> YVEFVAQISPQYPMFTVPLPIPPVKQPRLTVTNPVNGQEIWYYEVEIKPFTHQVYPDLGSADLVGYDGMSPGPTFQVPRGVETVVRFINNAEAPNSVHLHGSFSRAAFDGWAEDITEPGSFKDYYYPNRQSARTLWYHDHAMHITAENAYRGQAGLYMLTDPAEDALNLPSGYGEFDIPMILTSKQYTANGNLVTTNGELNSFWGDVIHVNGQPWPFKNVEPRKYRFRFLDAAVSRSFGLYFADTDAIDTRLPFKVIASDSGLLEHPADTSLLYISMAERYEVVFDFSDYAGKTIELRNLGGSIGGIGTDTDYDNTDKVMRFVVADDTTQPDTSVVPANLRDVPFPSPTTNTPRQFRFGRTGPTWTINGVAFADVQNRLLANVPVGTVERWELINAGNGWTHPIHIHLVDFKVISRTSGN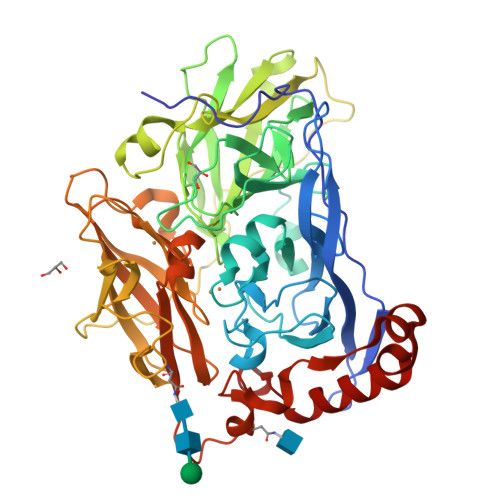NARTVMPYESGLKDVVWLGRRETVVVEAHYAPFPGVYMFHCHNLIHEDHDMMAAFNATVLPDYGYNATVFVDPMEELWQARPYELGEFQAQSGQFSVQAVTERIQTMAEYRPYAAADE>MPQSKSRKIAILGYRSVGKSSLTIQFVEGQFVDSYDPTIENTFTKLITVNGQEYHLQLVKTAGQDEYSIFPQTYSIDIN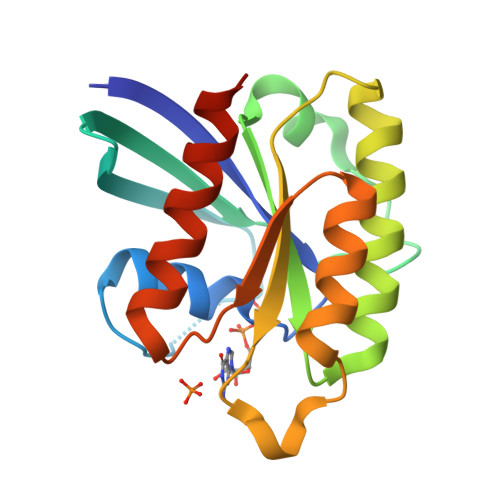GYILVYSVTSIKSFEVIKVIHGKLLDMVGKVQIPIMLVGNKKDLHMERVISYEEGKALAESWNAAFLESSAKENQTAVDVFRRIILEAEKLEHHHHHH[2x]> MAEEQARHVKNGLECIRALKAEPIGSLAIEEAMAAWSEISDNPGQERATCREEKAGSSGLSKPCLSAIGSTEGGAPRIRGQGPGESDDDAETLGIPPRNLQAS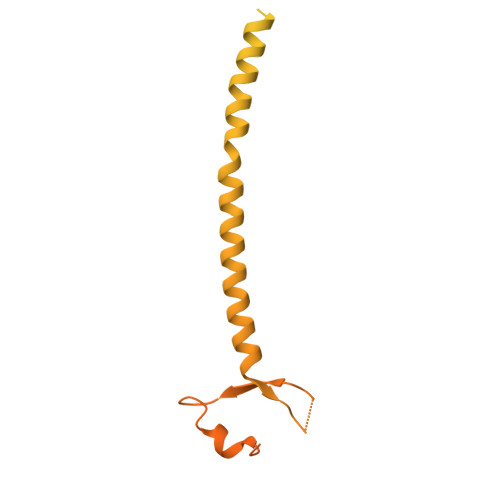STGLQCHYVYDHSGEAVKGIQDADSIMVQSGLDGDSTLSGGDNESENSDVDIGEPDTEGYAITDRGSAPISMGFRASDVETAEGGEIHELLRLQSRGNNFPKLGKTLNVPPPPDPGRASTSGTPIKKGTDARLASFGTEIASSLTGGATQCARKSPSEPSGPGAPAGNVPECVSNAALIQEWTPESGTTISPRSQNNEEGGDHYDDELFSDVQDIKTALAKIHEDNQKIISKLESLLLLKGEVESIKKQINRQNISISTLEGHLSSIMIAIPGLGKDPNDPTADVEINPDLKPIIGRDSGRALAEVLKKPVASRQLQGMTNGRTSSRGQLLKEFQLKPIGKKMSSAVGFVPDTGPASRSVIRSIIKSSRLEEDRKRYLMTLLDDIKGANDLAKFHQMLMKIIMKSG> MKRIGVLTSGGDSPGMNAAIRSVVRKAIYHGVEVYGVYHGYAGLIAGNIKKLEVGDVGDIIHRGGTILYT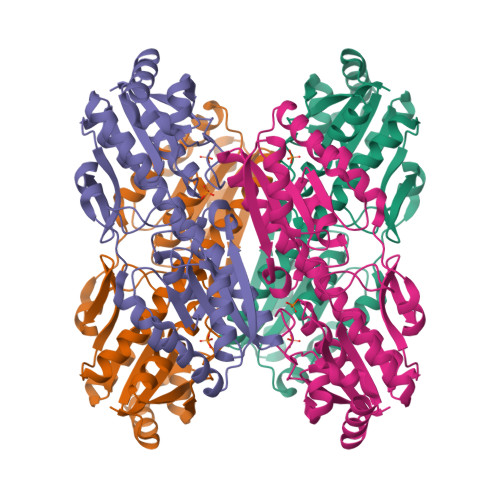ARCPEFKTEEGQKKGIEQLKKHGIQGLVVIGGDGSYQGAKKLTEHGFPCVGVPGTIDNDIPGTDFTIGFDTALNTVIDAIDKIRDTATSHERTYVIEVMGRHAGDIALWSGLAGGAETILIPEADYDMNDVIARLKRGHERGKKHSIIIVAEGVGSGVDFGRQIQEATGFETRVTVLGHVQRGGSPTAFDRVLASRLGARAVELLLEGKGGRCVGIQNNQLVDHDIAEALANKHTIDQRMYALSKELSI>MSLKQPLPEWQSQYAVGLNKLAPHTYVWPYADASDIGKPGGYEQSPYYMSLNGKWKFNWVKNPDNRPKDFYQPSYYTGGWADINVPGNWERQGYGTAIYVNETYEFDDKMFNFKKNPPLVPFAENEVGSYRRTFKVPADWKGRRVVLCCEGVISFYYVWVNGKLLGYNQGSKTAAEWDITDVLSEGENVVALEVYRWSSGAYLECQDMWRLSGIERDVYLYSTPKQYIADYKVSASLDKEKYKEGIFNLEVTVEGPSATASSIAYTLKDASGKAVLQDAINIKSRGLSNFIAFDEKKIAEVKAWNAEHPNLYTLVLELKDAQGKVTELTGCEVGFRTSEIKDGRFCINGVPVLVKGTNRHEHSQLGRTVSKELMEQDIRLMKQHNINMVRNSHYPTHPYWYQLCDRYGLYMIDEANIESHGMGYGPASLAKDSTWLTAHMDRTHRMYERSKNHPAIVIWSQGNEAGNGINFERTYDWLKSVEKGRPVQYERAELNYNTDIYCRMYRSVDEIKAYVGKKDIYRPFILCEYLHAMGNSCGGMKEYWEVFENEPMAQGGCIWDWVDQNFREIDKDGKWYWTYGGDYGPEGIPSFGNFCGNGLVNAVREPHPHLLEVKKIYQNIKATLSDRKNLKVCIKNWYDFSNLNEYILRWNVKGEDGTVLAEGTKEVDCEPHATVDVTLGAVKLPNTVREAYLNLSWSRKEATPLVDTDWEVAYDQFVLAGNKNTTAYRPQKAGETAFVVDKNTGALSSLTLDGKELLAAPITLSLFRPATDNDNRDRNGARLWRKAGLNNLTQKVVSLKEEKTSATVRAEILNGKGQKVGMADFVYALDKNGALKVRTTFQPDTAIVKSMARLGLTFRMADAYNQVSYLGRGDHETYIDRNQSGRIGLYDTTVERMFHYYATPQSTANRTDVRWAKLTDQAGEGVFMESNRPFQFSIIPFSDVLLEKAHHINELERDGMITIHLDA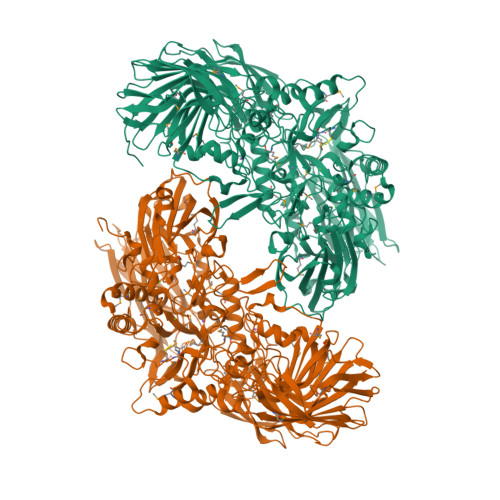EQAGVGTATCGPGVLPQYLVPVKKQSFEFTLYPVKEGHHHHHH[2x]[(3~{S},3~{a}~{S},8~{b}~{S})-3-(hydroxymethyl)-2,3,3~{a},8~{b}-tetrahydro-[1]benzofuro[3,2-b]pyrrol-1-yl]-phenyl-methanone 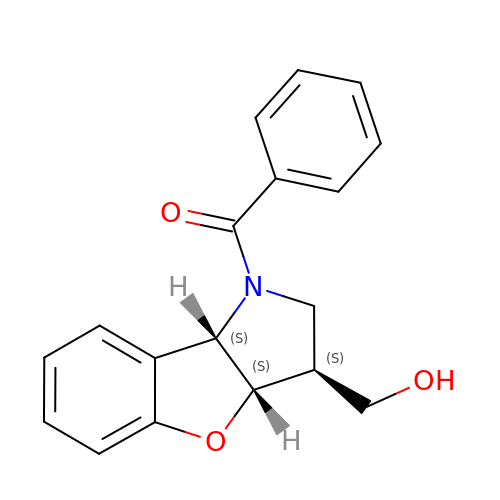| C18 H17 N O3 | VKQHNAPJGDBELB-JQFCIGGWSA-N2-amino-6-(5-fluoro-6-methoxypyridin-3-yl)-4-methyl-8-(pyrrolidin-1-yl)pyrido[2,3-d]pyrimidin-7(8H)-one 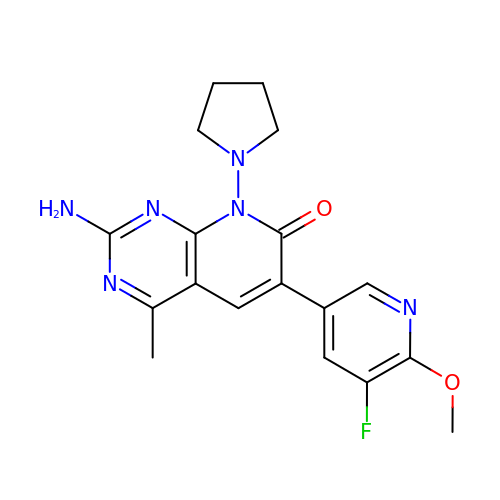| C18 H19 F N6 O2 | YJFBSFMYXTWDGD-UHFFFAOYSA-N2,2-dimethyl-1,3-dihydrobenzo[a]phenanthridin-4-one | C19 H17 N 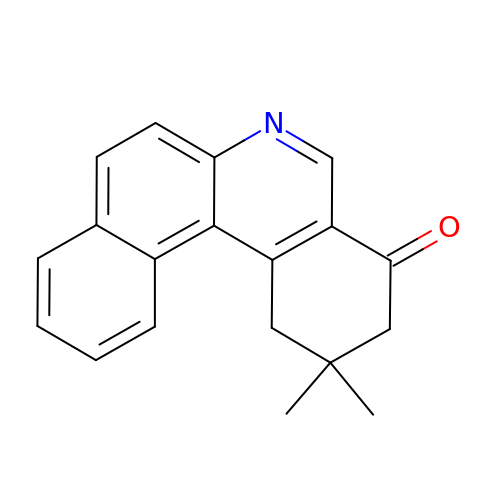O | VFHPHBGZIZTJDN-UHFFFAOYSA-N>[2x]GPHMRK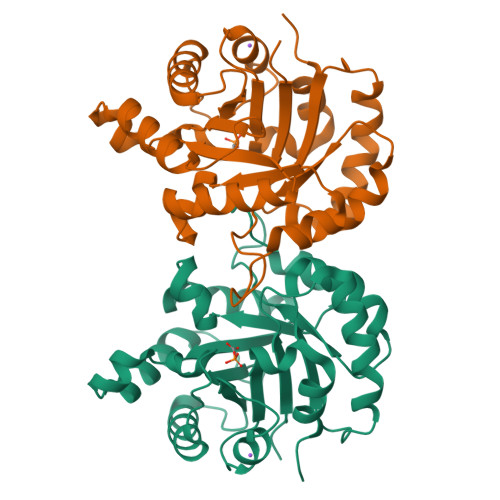IIIAGNWKMHKTQAEAQAFLQGFKPLIEDAAESREVVLCVPFTDLSGMSQQLHGGRVRLGAQNVHWEASGAYTGEISAAMLTEIGIHYVVIGHSERRQYFGETDETANLRVLAAQKAGLIPILCVGESKAQRDAGETEQVIVDQVKKGLVNVDQSNLVIAYEPIWAIGTGDTCAATEANRVIGLIREQLTNSQVTIQYGGSVNANNVDEIMAQPEIDGALVGGASLEPQSFARIVNFQP~{N}-[2-chloranyl-5-(3,6-dihydro-2~{H}-pyran-4-yl)pyridin-3-yl]methanesulfonamide | C11 H13 Cl N2 O3 S | 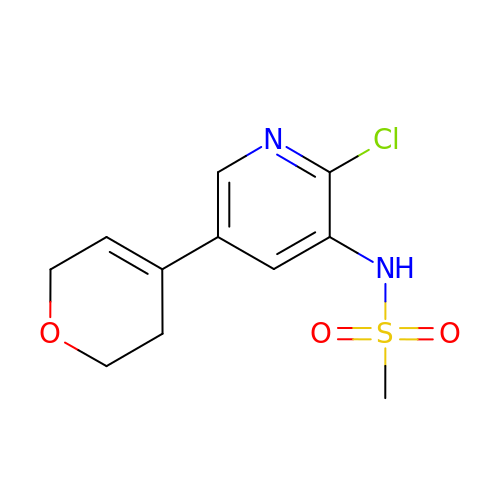PGVPPOVJVOILFT-UHFFFAOYSA-N> MPAIMTMLADHAARQLLDFSQKLDINLLDNVVNCLYHGEGAQQRMAQEVLTHLKEHPDAWTRVDTILEFSQNMNTKYYGLQILENVIKTRWKILPRNQCEGIKKYVVGLIIKTSSDPTCVEKEKVYIGKLNMILVQILKQEWPKHWPTFISDIVGASRTSESLCQNNMVILKLLSEEVFDFSSGQITQVKSKHLKDSMCNEFSQIFQLCQFVMENSQNAPLVHATLETLLRFLNWIPLGYIFETKLISTLIYKFLNVPMFRNVSLKCLTEIAGVSVSQYEEQFVTLFTLTMMQLKQMLPLNTNIRLAYSNGKDDEQNFIQNLSLFLCTFLKEHDQLIEKRLNLRETLMEALHYMLLVSEVEETEIFKICLEYWNHLAAELYRESPFSTSASPLLSGSQHFDVPPRRQLYLPMLFKVRLLMVSRMAKPEEVLVVENDQGEVVREFMKDTDSINLYKNMRETLVYLTHLDYVDTERIMTEKLHNQVNGTEWSWKNLNTLCWAIGSISGAMHEEDEKRFLVTVIKDLLGLCEQKRGKDNKAIIASNIMYIVGQYPRFLRAHWKFLKTVVNKLFEFMHETHDGVQDMACDTFIKIAQKCRRHFVQVQVGEVMPFIDEILNNINTIICDLQPQQVHTFYEAVGYMIGAQTDQTVQEHLIEKYMLLPNQVWDSIIQQATKNVDILKDPETVKQLGSILKTNVRACKAVGHPFVIQLGRIYLDMLNVYKCLSENISAAIQANGEMVTKQPLIRSMRTVKRETLKLISGWVSRSNDPQMVAENFVPPLLDAVLIDYQRNVPAAREPEVLSTMAIIVNKLGGHITAEIPQIFDAVFECTLNMINKDFEEYPEHRTNFFLLLQAVNSHCFPAFLAIPPTQFKLVLDSIIWAFKHTMRNVADTGLQILFTLLQNVAQEEAAAQSFYQTYFCDILQHIFSVVTDTSHTAGLTMHASILAYMFNLVEEGKISTSLNPGNPVNNQIFLQEYVANLLKSAFPHLQDAQVKLFVTGLFSLNQDIPAFKEHLRDFLVQIKEFAGEDTSDLFLEEREIALRQADEEKHKRQMSVPGIFNPHEIPEEMCD;> SMEELSQALASSFSVSQDLNSTAAPHPRLSQYKSKYSSLEQSERRRRLLELQKSKRLDYVNHARRLAEDDWTGMESEEENKKDDEEMDIDTVKKLPKHYANQLMLSEWLIDVPSDLGQEWIVVVCPVGKRALIVASRGSTSAYTKSGYCVNRFSSLLPGGNRRNSTAKDYTILDCIYNEVNQTYYVLDVMCWRGHPFYDCQTDFRFYWMHSKLPEEEGLGEKTK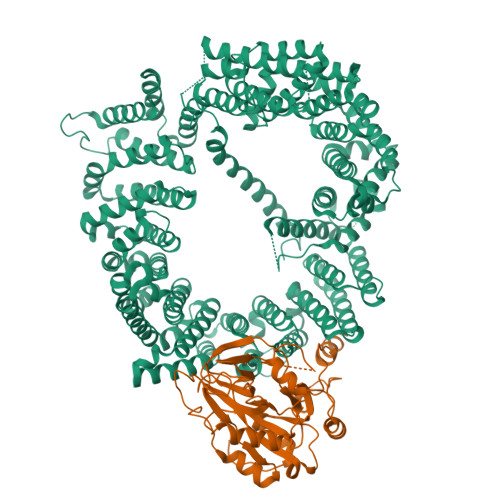LNPFKFVGLKNFPCTPESLCDVLSMDFPFEVDGLLFYHKQTHYSPGSTPLVGWLRPYMVSDVLGVAVPAGPLTTKPDYAGHQLQQIMEHKKSQKEGMKEKLTHKA>[2x]MATSMTDIKGFNMISIEQEKELGNKFAVEIEKQQQPVNDPEVQRYVDKVGKRLLSGARAVEFDYVFKVVKDDSVNAFAIPGGRVYVHTGLLKAADNETELAGVLAHEINHAVARHGTR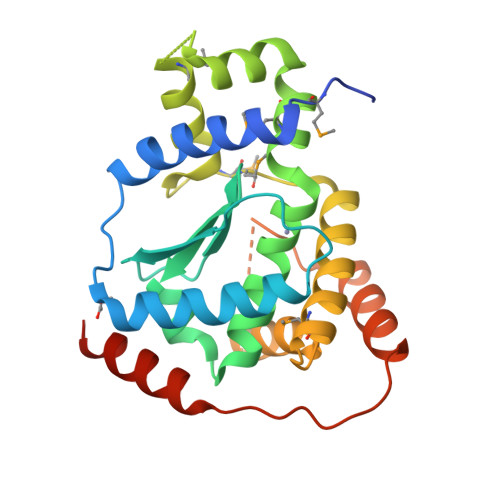QMTQEYGYSLVLSLVLGDNPNMLAQLAGQLFGKAGMMSYSREYENQADFLGVETMYKAGYNPNGLTSFFQKLNAMDGGTQSNVARFFSTHPLTSERIQRVQAEIAKLPPQRYLTDETEFKKIKGRLKLEHHHHHH Members of the family Birnaviridae possess bi-segmented double-stranded RNA (dsRNA) genomes and form virions with non-enveloped single-shelled icosahedral capsids. From sequence analysis it was proposed that the RdRPs of Birnaviridae possess a non-canonical active site where the polymerase sequence motifs are re-ordered C-A-B, motif C containing ADN in place of the conserved GDD catalytic residues. An additional unusual feature of birnavirus RdRPs is their ability to self-guanylylate: auto-catalyzing the covalent addition of a GMP moiety to a serine residue of the polymerase in a template-independent manner to form VP1pG. We have cloned, expressed and solved the structure of the RdRP VP1 from IPNV in both its apo form and bound to a catalytic metal (magnesium).

Clear electron density connects the helix with residue 31 of an adjacent molecule in the crystal in 7 of the 8 molecules present in the asymmetric unit. In addition, residues 3–10 are seen in this structure extending toward the catalytic active site. As in the high-resolution structures, the helix formed by residues 13–19 lies in a hydrophobic pocket within the active site cleft formed by loops of the fingers domain and the N-terminal extension. Residues 11–12 form a short isolated β strand which interacts with residue 241 of the fingers domain, while residue 10 spans the two sides of the active site cleft. Residues 7–10 interact with a loop between residues 594–598 of the thumb, this loop being partly mobile and modeled as having two conformations in the refined structure. Residues 3–6 interact with the thumb, the palm and the C-terminal extension, the side chain of F5 being buried in a hydrophobic pocket between the side chains of residues W563, L578, R582 and F662. While the conformation of S2 (the first residue of mature VP1 assuming removal of the initiator methionine by methionine aminopeptidase) could not be assigned unambiguously, it will clearly lie extremely close to the catalytic residues of the active site. The observed self-interaction brings the N-terminal residue of VP1 (S2, assuming removal of the initiator methionine) within approximately 5 Å of the catalytic site, and removal of the N-terminal tail or mutation of S2 to alanine abolishes the ability of VP1 to form covalent RNA∶polymerase complexes. Instead, we propose that residue S2 at the N-terminus of VP1 represents the site of covalent attachment of RNA product to the polymerase.

>MSDIFNSPQNKASILTALMKSTTGDVEDVLIPKRFRPAKDPLDSPQAAAQFLKDNKYRILRPRAIPTMVELETDAALPRLRQMVEDGKLKDTVSVPEGTTAFYPKYYPFHKPDHDEVGTFGAPDITLLKQLTFFLLENDFPTGPETLRQVREAIATLQYGSGSYSGQLNRLLAMKGVATGRNPNKTPKTVGYTNEQLAKLLEQTLPINTPKHEDPDLRWAPSWLINYTGDLSTDKSYLPHVTIKSSAGLPYIGKTKGDTTAEALVLADSFIRDLGRAATSADPEAGVKKTITDFWYLSCGLLFPKGERYTQVDWDKKTRNIWSAPYPTHLLLSMVSTPVMNESKLNITNTQTPSLYGFSPFHGGMDRIMTIIRDSLDNDEDLVMIYADNIYILQDNTWYSIDLEKGEANCTPQHMQAMMYYLLTRGWTNEDGSPRYNPTWATFAMNVAPSMVVDSSCLLMNLQLKTYGQGSGNAFTFLNNHLMSTIVVAEWVKAGKPNPMTKEFMDLEEKTGINFKIERELKNLRETIVEAVETAPQDGYLADGSDLPPIRPGKAVELDLLGWSAIYSRQMEMFVPVLENERLIASAAYPKGLENKALARKPGAEIAYQIVRYEAIRLVGGWNNPLLETAAKHMSLDKRKRLEVKGIDVTGFLDDWNNMSEFGGDLEGITLSEPLTNQTLVDINTPLDSFDPKARPQTPRSPKKTLDEVTTAITSGTYKDPKSAVWRLLDQRTKLRVSTLRDQALALKPASSSVDNWAEATEELAQQQQLLMKANNLLKSSLTETREALEKTGHHHHHH[8x]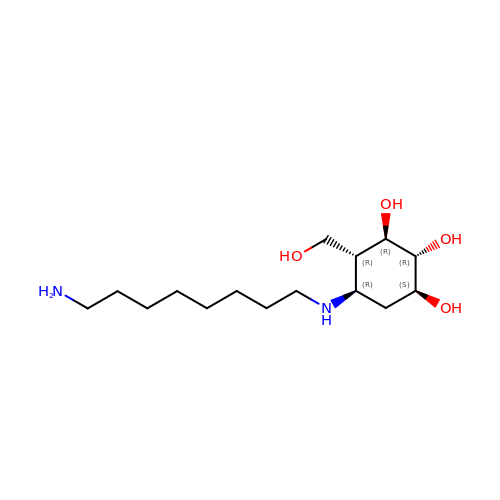(1~{S},2~{R},3~{R},4~{R},5~{R})-5-(8-azanyloctylamino)-4-(hydroxymethyl)cyclohexane-1,2,3-triol | C15 H32 N2 O4 | HEJOCOWXPPQFHY-XPABHHOTSA-N> MQSPPGKPEIHKCRSPDKETFTCWWNPGTDGGLPTNYSLTYSKEGEKTTYECPDYKTSGPNSCFFSKQYTSIWKIYIITVNATNQMGSSSSDPLYVDVTYIVEPEPPRNLTLEVKQLKDKKTYLWVKWSPPTITDVKTGWFT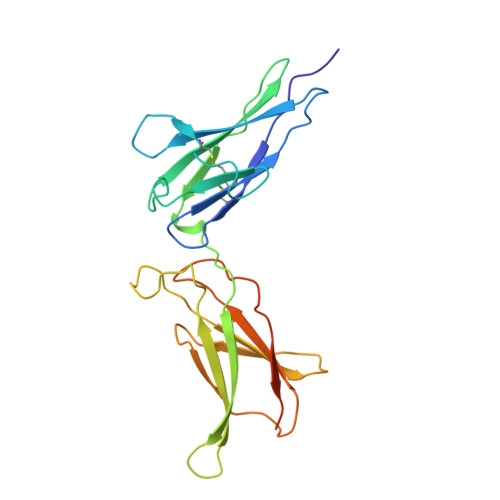MEYEIRLKPEEAEEWEIHFTGHQTQFKVFDLYPGQKYLVQTRCKPDHGYWSRWSQESSVEMPNDFTLKDRSRSHHHHHH>MSLQPFFGFPPTVNDLFSDFVSYSPRLNNQIPGELSPSIDVHEGKDTVSVDVELPGVKKEDVQVHYDSG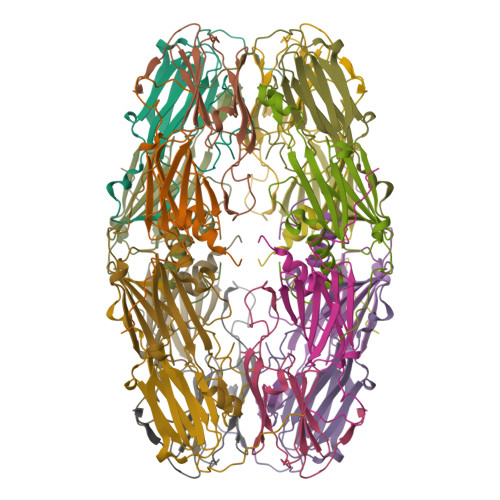KLTISGEVVNERKNESTEGNQRWSERRFGSFSRTITIPAKIDADRIEANFSNGLLTVTLPKVEKSQTKKQIAIK[4x]>[3x]MMMASKDATSSVDGASGAGQLVPEVNASDPLAMDPVAGSSTAVATAGQVNPIDPWIINNFVQAPQGEFTISPNNTPGDVLFDLSLGPHLNPFLLHLSQMYNGWVGNMRVRIMLAGNAFTAGKIIVSCIPPGFGSHNLTIAQATLFPHVIADVRTLDPIEVPLEDVRNVLFHNNDRNQQTMRLVCMLYTPLRTGGGTGDSFVVAGRVMTCPSPDFNFLFLVPPTVEQKTRPFTLPNLPLSSLSNSRAPLPISSMGISPDNVQSVQFQNGRCTLDGRLVGTTPVSLSHVAKIRGTSNGTVINLTELDGTPFHPFEGPAPIGFPD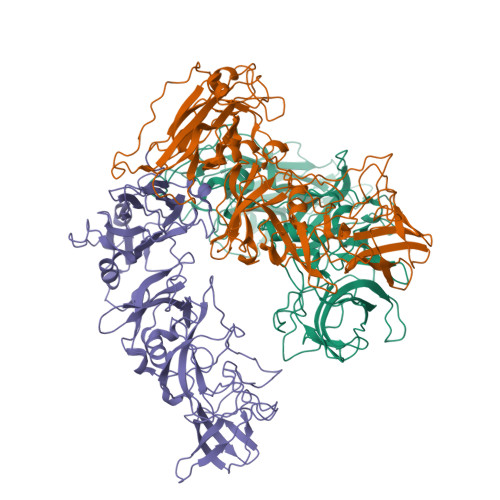LGGCDWHINMTQFGHSSQTQYDVDTTPDTFVPHLGSIQANGIGSGNYVGVLSWISPPSHPSGSQVDLWKIPNYGSSITEATHLAPSVYPPGFGEVLVFFMSKMPGPGAYNLPCLLPQEYISHLASEQAPTVGEAALLHYVDPDTGRNLGEFKAYPDGFLTCVPNGASSGPQQLPINGVFVFVSWVSRFYQLKPVGTASSARGRLGLRR Brigimadlin | C31 H25 Cl2 F N4 O3 | 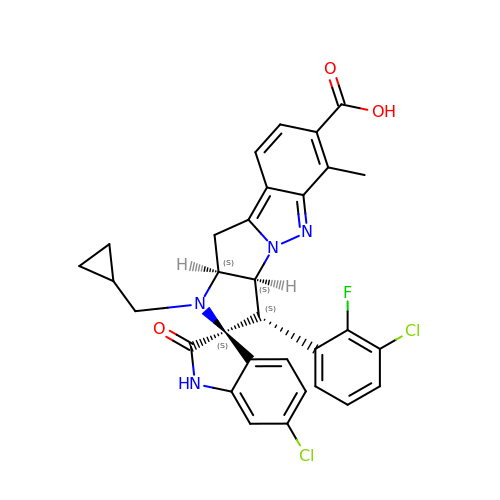AMTXDBGKYPDTTA-SJVQGLCSSA-N> HHHHHHHHPPSGADPMYAMPGNSGDLQCDDGKKRHIPPLSLLLSGYGSSEGRELDTSYTPKQWLWFLYVTSWARPFFTYASSGGASEATEGSSDNRSGSAYWGRLSFDELLKLSGSPIPPAMVSLWMGLCMPTDDVVQELRIMTEGKAEGRQRIYPFLPRVAESTFGRALRSLAVRQHISSWMPSHAGDVCAALDVLVRDTLEVIQNSADVRKTARVRCEERDASGEEALEGAFRSMLSASTTAPKVVEATTYRPLFDVKASIPEGGTAQVLIRVANAARLFAALSVEAFGRVKSECAVLLLAHINQRDAPEHVDARAYGVVTGVVEYAMAYRYCRDDGTGRCPLTCAALLLHRLVELQGIVEKDTAAGDRCMGMAVSASRFANMTVACIQELLFCVVAGDTVRWHREHQPDGVSVCPTAARTLTLHETDCLLQVFIPALLQQVGFEWPWSESLRHAKMLDRARTQHIVMEDGVRLDSRSVFEELLVSVARRTYGLRLRAILPQSFDVIAENIFVSIHDVPNEGKSSGGNPEKVADNSSSRFALPLYYRTAGEVLLEYFDRCGPSGITAEETERVLRRATDVQPMVVQLQALGGDTNGGITDCVSYCGELSRTVYFSAREKERLLQRYRCEVLLASLVVYTQLRTVSVVQQLTRQLAPLFEQLLLPLAHERTLSRCPVIASRKGDGVDDNGTPLVDLTPEFKMLVDEIHYEFYPLEWVPEAVDAHIRQECGVREKEGAPYHEGGNGPPCFAQYSLFAAIAHQFGLVLEGNPRGFRGGDGSSSEVRTKAYRFFTLMLLNNLGDAVSSSCELDGAAALAATRRVKDCQDGSENCKQRQAAVRQRGGASFHSVVSACDVVVTMTQCLLPAHLSSHPRMATTGSMSNEWMRRVGEWTRSAYSKYTAYQQQVHGLDLPVPLISLYNSLTFDSVPLARETIRAVRSRLLEKMSVVTASPPGDVETAGKQLLEQHLSSLTVTLTAVGLLPLCVRGGSHVPCATQLLWASPFFSHELLHCGRYEVSV;> MAEYLIDLTPRMAYVDRHELLRSLLTEKEFIERRQEQLNKSTTVYVGNLSFYTTEDQIWEHFSRCGHIRDLVMGLSEVTRTPCGFCFVVFESQDGAMSAVIDLHGTLLDDRVITVSWDVGCDHTRRWGRGAHGGQVVDGVRQNLDSARGGLGVLRREELGVGAAVAEDQLVHYTWIPPRRVEKRGRS;> MRRGSGFVHLNTPAAISYSPGQQVSLSDLRQKRRREECVVLPPIMTVWRSAFSQYTKMWGLTKFAGDIEAEREGEGPILPPIREETVVKSTTHSFKGKSTTVAAAVATPPGEKGIEIVSHHKLCGKQRFVYPDHDGVLSSGIVPKVV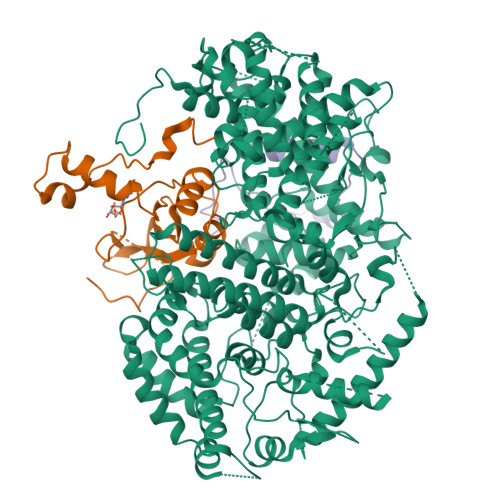ISKEEEEEMEANKKYYISPQEMTEEERNAFEELDAMWKSYARGRSEQGARHRAFAGTVTPGDAMTEVEEETGNNRGNARRRLESHTPRQHPQESAAEGNSVAHNTEEALDDALRLIDELLEFN> VGAITTIEDPVLA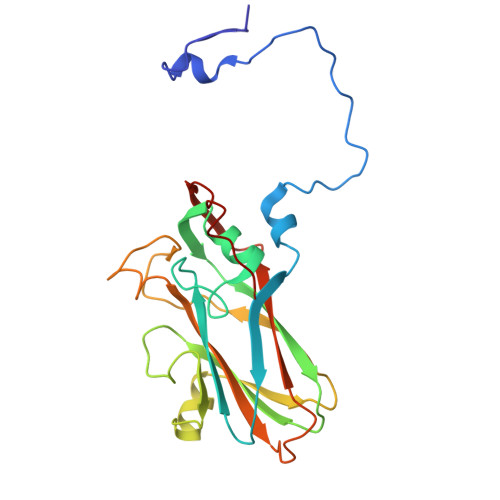KKVPETFPELKPGESRHTSDHMSIYKFMGRSHFLCTFTFNSNNKEYTFPITLSSTSNPPHGLPSTLRWFFNLFQLYRGPLDLTIIITGATDVDGMAWFTPVGLAVDTPWVEKESALQIDYKTALGAVRFNTRRTGNIQIRLPWYSYLYAVSGALDGLGDKTDSTFGLVSIQIANYNHSDEYLSFSCYLSVTEQSEFYFPRAPLNSNAMLST>[2x]MCGIFAYLNYHVPRTRREILETLIKGLQRLEYRGYDSAGVGFDGGNDKDWEANACKIQLIKKKGKVKALDEEVHKQQDMDLDIEFDVHLGIAHTRWATHGEPSPVNSHPQRSDKNNEFIVIHNGIITNYKDLKKFLESKGYDFESETDTETIAKLVKYMYDNRESQDTSFTT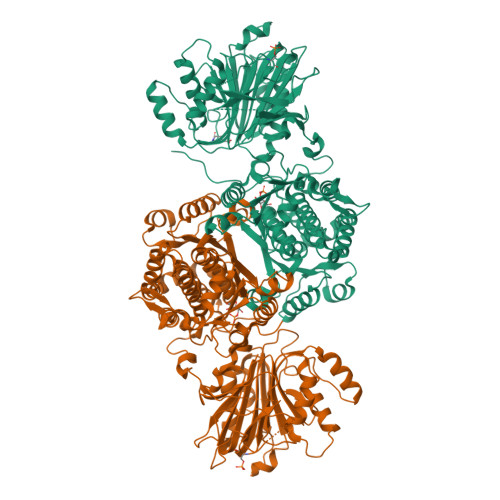LVERVIQQLEGAFALVFKSVHFPGQAVGTRRGSPLLIGVRSEHKLSTDHIPILYRTGKDKKGSCNLSRVDSTTCLFPVEEKAVEYYFASDASAVIEHTNRVIFLEDDDVAAVVDGRLSIHRIKRTAGHHHHHHDHPGRAVQTLQMELQQIMKGNFSSFMQKEIFEQPESVVNTMRGRVNFDDYTVNLGGLKDHIKEIQRCRRLILIACGTSYHAGVATRQVLEELTELPVMVELASDFLDRNTPVFRDDVCFFLSQSGETADTLMGLRYCKERGALTVGITNTVESSISRETDCGVHINAGPEIGVASTKAYTSQFVSLVMFALMMCDDRISMQERRKEIMLGLKRLPDLIKEVLSMDDEIQKLATELYHQKSVLIMGRGYHYATCLEGALKIKEITYMHSEGILAGELKHGPLALVDKLMPVIMIIMRDHTYAKCQNALQQVVARQGRPVVICDKEDTETIKNTKRTIKVPHSVDCLQGILSVIPLQLLAFHLAVLRGYDVDFPRNLAKSVTVE>GMTQDNASGDQVSKQHKAFLRKLYLAHLMDDARHNLLSLGKLTGMPRRTLQDAIASFADIGIEVEFVQDGERHNAGYYRIRTWGPISSAWMDTHVDEV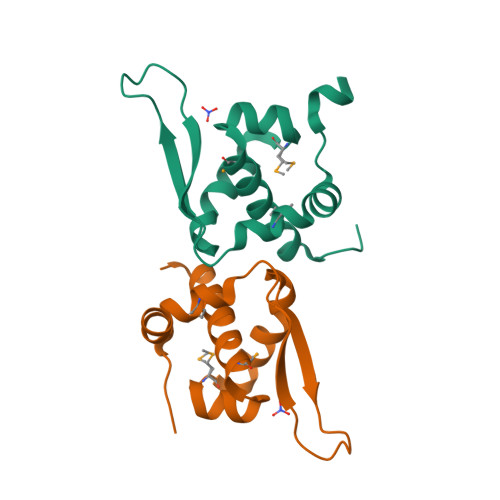KSLLGVDDAVGQATAGNGA[3x]>MSRVLLCSAGHSSMVVPEAFHAVPEGFEEVHVFTTDSEKFNPVVLNDFFHSLPNVRFSITKCHGLADILNERDFEFYQEMLWQWYLTKMPDNELPYVCLSGGIKSMSASLQKAATLFGAQSVFHVLADNNPRNIEEMFDALQKGQIHFIEMGYEPGWAALRRLKKILPINEGCSRDNFKPLISKSIEEILSNVKIMASDTGKSNQLPFPSLAILPPIAQQWLQLPLSANDGAWIQNLPKVDLHCHLGGFATSGSLLDQVRGAASEPDLIDRTFSPQEIAGWPRSHKSISLDKYMELGNANGSKLLKDKGCLIRQVELLYQSLVNDNVAYAEIRCSPNNYADKNKNRSAWVVLQDINDTFTRLITEAKQKNQFYCHVNLLVIASRKFSGDLSDISKHLALAITAMQQGEGVCRIVGVDLAGFENKETRASYYEHDFKAVHRCGLAVTAHAGENDDPEGIWQAVYSLHARRLGHALNLLEAPDLMRTVIERKIGVEMCPYANYQIKGFAPMPNFSALYPLKKYLEAGILVSVNTDNIGISGANLSENLLILADLCPGISRMDVLTIIRNSIETAFISHDFRMELLKFFDRKIYDVCLISIKN[6x]

In order to identify novel CARF effectors, we used Foldseek18 to search for proteins with structural homology to CARF domain of the Cam1 effector. This method rendered a 600-residue protein containing an N-terminal CARF domain followed by a linker region and a C-terminal adenosine deaminase (ADA) domain, with accession number HAJ98955.1 from an unknown Bacteriodales bacterium (hereafter named CRISPR-associated deaminase, CRISPR-associated adenosine deaminase 1 [Cad1]), for which homologs were already identified in a previous bioinformatic screen. cad1 is located immediately downstream the cas10-csm genes of a type III-A CRISPR locus. Further analysis of cad1 homologs showed that over 70% associate in genomes containing type III systems (mostly belonging to the A and B subtypes) and exist within many unique phyla of bacteria. These data suggest that Cad1 is a widespread effector in type III CRISPR-Cas systems. Altogether, these data demonstrate that Cad1 deaminates ATP molecules to ITP through the formation of an hexameric complex that requires a Mg+2 or Mn+2 cofactor and an activating cA4 or cA6 ligand. While the triggering of a growth arrest in the host is a common strategy of all CARF effectors, we believe that Cad1 introduces a new mode of defense for CRISPR-Cas systems that couples nucleotide deamination activity to a sequence-specific, RNA-guided adaptive immune response.

First, we used SECMALS to analyze the oligomeric state of the protein and found that the majority of Cad1 forms a hexameric (403 kDa ± 0.451%) species in solution, with a small amount of the dimeric (139 kDa ± 1.1%) species and of a higher molecular weight (5–31 MDa) megadalton fraction (peaks “H, ” “D, ” and “M, ” respectively). To understand the organization of the protein at the atomic level, we solved the cryoelectron microscopy (cryo-EM) structure of hexameric apo-Cad1 at 3.6 Å resolution. Consistent with the SECMALS data, the structure displayed a trimeric arrangement of Cad1 dimers forming a homohexamer. The dimeric deaminase domains form the core of the hexamer by arranging themselves with 3-fold symmetry and are linked to the CARF head domains through a 51-amino-acid linker (L1, inset). Further, we observed that the dimeric CARF head groups are tilted to one side with respect to a vertical axis from the center of 3-fold symmetry (black dotted arrows). The tilting of the CARF domain around the L1 linker brings it close to the deaminase domain on one side and distant from the deaminase domain at the opposite side (labeled as “closed” and “open, ” red arrows). On the other hand, mutation of W349, which interacts with its counterpart in another Cad1 dimer via π-π stacking of aromatic rings (inset), led to the detection of a stable dimeric complex by SECMALS.> MAFSKLLEQAGGVGLFQTLQVLTFILPCLMIPSQMLLENFSAAIPGHRCWTHMLDNGSAVSTNMTPKALLTISIPPGPNQGPHQCRRFRQPQWQLLDPNATATSWSEADTEPCVDGWVYDRSVFTSTIVAKWDLVCSSQGLKPLSQSIFMSGILVGSFIWGLLS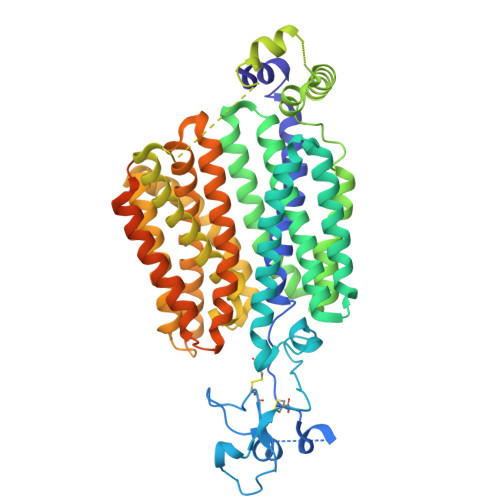YRFGRKPMLSWCCLQLAVAGTSTIFAPTFVIYCGLRFVAAFGMAGIFLSSLTLMVEWTTTSRRAVTMTVVGCAFSAGQAALGGLAFALRDWRTLQLAASVPFFAISLISWWLPESARWLIIKGKPDQALQELRKVARINGHKEAKNLTIEVLMSSVKEEVASAKEPRSVLDLFCVPVLRWRSCAMLVVNFSLLISYYGLVFDLQSLGRDIFLLQALFGAVDFLGRATTALLLSFLGRRTIQAGSQAMAGLAILANMLVPQDLQTLRVVFAVLGKGCFGISLTCLTIYKAELFPTPVRMTADGILHTVGRLGAMMGPLILMSRQALPLLPPLLYGVISIASSLVVLFFLPETQGLPLPDTIQDLESQKSTAAQGNRQEAVTVESTSLHHHHHHHHHHGSVEDYKDDDDK> MVVFEITILGANGGPTEYGTQCFILKPARTEDPELIAVDGGAGMYQLREMLVQGRNENEGDDELVPSFYEHDREPIEFFIDSKLNIQKGLSKSLLQSLKRQGEHFESANTMKKTYEVFQGITDYYITHPHLDHI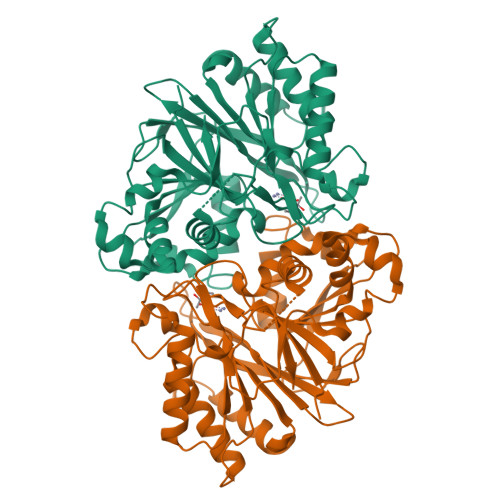SGLVVNSPSIYEQENSKKKTIWGLPHTIDVLQKHVFNDLIWPDLTAERSRKLKLKCLNPKEVQKCTIFPWDVIPFKVHHGIGVKTGAPVYSTFYIFRDRKSKDCIIVCGDVEQDRRESEESLLEEFWSYVAENIPLVHLKGILVECSCPLSSKPEQLYGHLSPIYLINELSNLNTLYNSSKGLSGLNVIVTHVKSTPAKRDPRLTILEELRFLAEERNLGDLRISIALEGHTLFL N-[1-(5-{[2-(4-FLUOROPHENOXY)ETHYL]SULFANYL}-4-METHYL-4H-1,2,4-TRIAZOL-3-YL)ETHYL]-2-(TRIFLUOROMETHYL)BENZAMIDE | 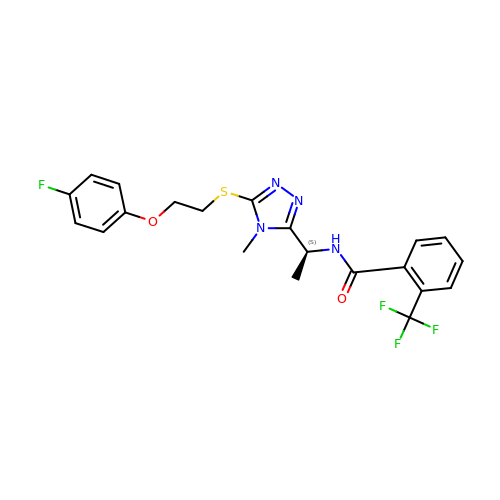C21 H20 F4 N4 O2 S | MFAPRDBSWRWQBP-ZDUSSCGKSA-N>SEMTPREIVSELDKHIIGQDNAKRSVAIALRNRWRRMQLNEELRHEVTPKNILMIGPTGVGKTEIARRLAKLANAPFIKVEATKFTEVGYVGKEVDSIIRDLTDAAVKMVRVQAIEKNRYRAEELAEERILDVLIPPAKNNWGQTEQQQEPSAARQAFRKKLREGQLDDKEIEIDLAAAPMGVEIMAPPGMEEMTSQLQSMFQNLGGQKQKARKLKIKDAMKLLIEEEAAKLVNPEELKQDAIDAVEQHGIVFIDEIDKICKRGESSGPDVSREGVQRDLLPLVEGCTVSTKHGMVKTDHILFIASGAFQIAKPSDLIPELQGRLPIRVELQALTTSDFERILTEPNASITVQYK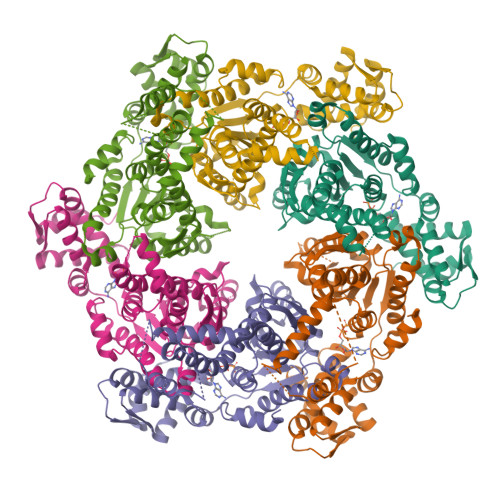ALMATEGVNIEFTDSGIKRIAEAAWQVNESTENIGARRLHTVLERLMEEISYDASDLSGQNITIDADYVSKHLDALVADEDLSRFIL[24x]>SNAQLTFQTSSPAHLTMPYVMPGDGEVVGVGEPVAIRFDENIADRGAAEKAIKITTNPPVEGAFYWLNNREVRWRPEHFWKPGTAVDVAVNTYGVDLGEGMFGEDNVQTHFTIGDEVIATADDNTKILTVRVNGEVVKSMPTSMGKDSTPTANGIYIVGSRYKHIIMDSSTYGVPVNSPNGYRTDVDWATQISYSGVFVHSAPWSVGAQGHTNTSHGCLNVSPSNAQWFYDHVKRGDIVEVVNTVGGTLPGIDGL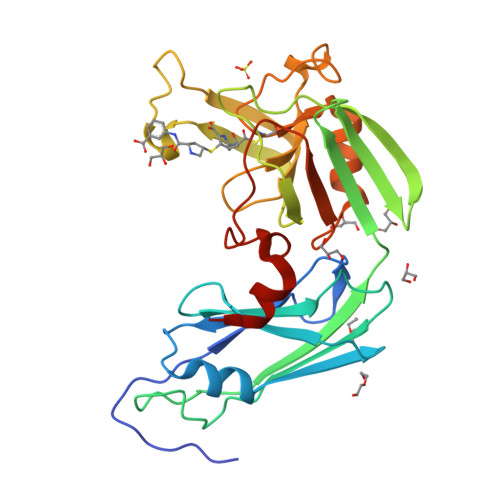GDWNIPWDQWRAGNAKA[2x]N'-[(2S,3S)-3-hydroxy-1-phenyl-4-{[2-(pyridin-2-yl)propan-2-yl]amino}butan-2-yl]-N,N-dipropyl-5-(pyridin-1(2H)-yl)benzene-1,3-dicarboxamide 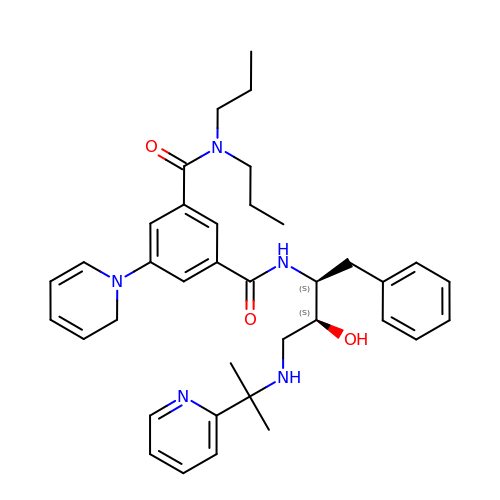| C37 H47 N5 O3 | BUOYUEMVUCMLPE-LQJZCPKCSA-N> MPRGSALSDTERAQLDVMKLLNVSLHEMSRKISRSRHCIR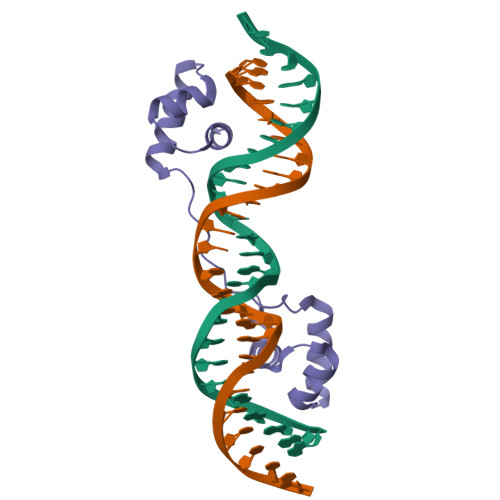VYLKDPVSYGTSKRAPRRKALSVRDERNVIRAASNSCKTARDIRNELQLSASKRTILNVIKRSGVIVRQKLRPAPLLSADHKLKRLEFAKNNMGTHHHHHH> SSGT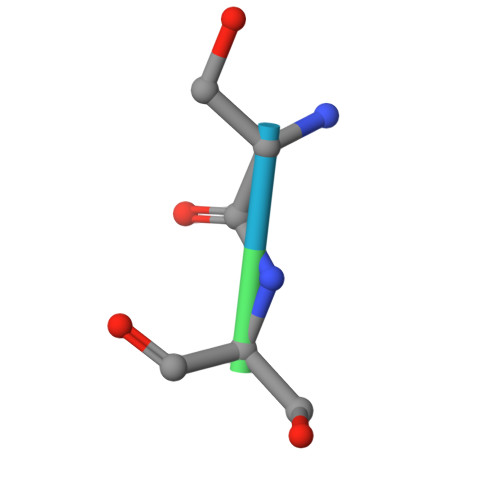PT> MPSIAFSGISTKPGELEFHVPSVLSKHNRAGLLKSIDFPYSQRTIESSWNKLHYMESIRITPESRSVSVLLTDKESGDRVEMLAMVPLTTNKIIEISTATTDGTIILVTEEPHGFFAPGCFGKEVRNVISSYKSIFPHGTPPFILIHGSNGSVQVDPALFEYNDEYSVKIKYTAIRTEFKLFGKGDHGWMV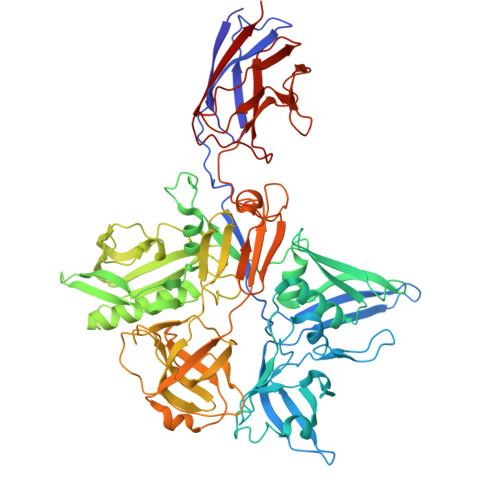TPEFPTISMLCQVITNAMNSAIIFNHDDPAARTRMYPGTCSNTHVIESVSGDSLAKALLGYDGVYAGWEEITIPAGMYCYGELDLSKMIAAKMNRWHIDRESSIIFRGVSGYTWNVTLPSGNYGTPEKLAHCIQHMMNMTAKNRKNPYCVRFTLNEGSSHRGKFVFVAAEPFDLLFGDDESIDPSILGFEPVDHIGRNSYMSENDLGAPLMKPNCNVYDVDEIPGTHQIRIGRRTRLAVDGKIRGYSGGTLRLNTVNRTTGAPKCHGMNKGDVVTLTTVMPAPDGATGTKREGFTFRAKNKIMGVVVADENENPDASSLHVSVPSMSWTLGIGSYITIDSQAAPISVALFDPGKNQFFRDSIGASRLGFSNGVSTGQHGVVVSQCAVNLEPRTVDVSFIEGSMTSASTEMYNQNGKSLITQVPSDRSSGPVPQGMVRFNNALQQFKLEFTNPDGSPYHFNHASLSLLMEFDD> MQGSVTEFLKPRLVDIEQVSSTHAKVTLEPLERGFGHTLGNALRRILLSSMPGCAVTEVEIDGVLHEYSTKEGVQEDILEILLNLKGLAVRVQGKDEVILTLNKSGIGPVTAADITHDGDVEIVKPQHVICHLTDENA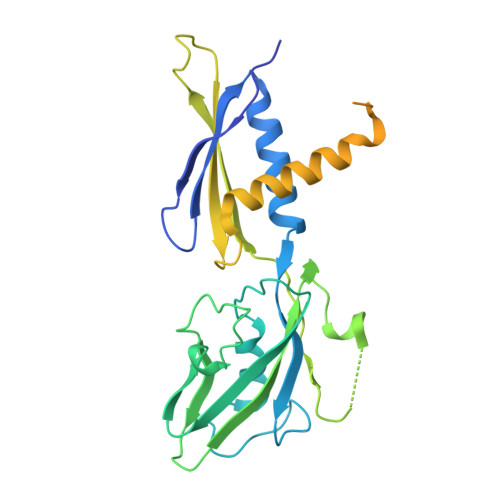SISMRIKVQRGRGYVPASTRIHSEEDERPIGRLLVDACYSPVERIAYNVEAARVEQRTDLDKLVIEMETNGTIDPEEAIRRAATILAEQLEAFVDLRDVRQPEVKEEKPEFDPILLRPVDDLELTVRSANCLKAEAIHYIGDLVQRTEVELLKTPNLGKKSLTEIKDVLASRGLSLGMRLENWPPASIADE> APDTSVSNKQNFSTDVIYQIFTDRFSDGNPANNPTGAAFDGTCTNLRLYCGGDWQGIINKINDGYLTGMGVTAIWISQPVENIYSIINYSGVNNTAYHGYWARDFKKTNPAYGTIADFQNLIAAAHAKNIKVIIDFAPNHTSPASSDQPSFAENGRLYDNGTLLGGYTNDTQNLFHHNGGTDFSTTENGIYKNLYDLADLNHNNSTVDVYLKDAIKMWLDLGIDGIRMDAVKHMPFGWQKSFMAAVNNYKPVFTFGQWFLGVNEVSPENHKFANESGMSLLDFRFAQKVRQVFRDNTDNMYGLKAMLEGSAA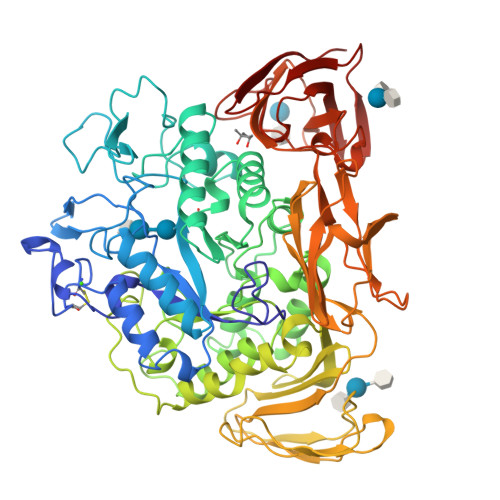DYAQVDDQVTFIDNHDMERFHASNANRRKLEQALAFTLTSRGVPAIYYGTEQYMSGGTDPDNRARIPSFSTSTTAYQVIQKLAPLRKSNPAIAYGSTQERWINNDVLIYERKFGSNVAVVAVNRNLNAPASISGLVTSLPQGSYNDVLGGLLNGNTLSVGSGGAASNFTLAAGGTAVWQYTAATATPTIGHVGPMMAKPGVTITIDGRGFGSSKGTVYFGTTAVSGADITSWEDTQIKVKIPAVAGGNYNIKVANAAGTASNVYDNFEVLSGDQVSVRFVVNNATTALGQNVYLTGSVSELGNWDPAKAIGPMYNQVVYQYPNWYYDVSVPAGKTIEFKFLKKQGSTVTWEGGSNHTFTAPSSGTATINVNWQP>HHHHHHGSM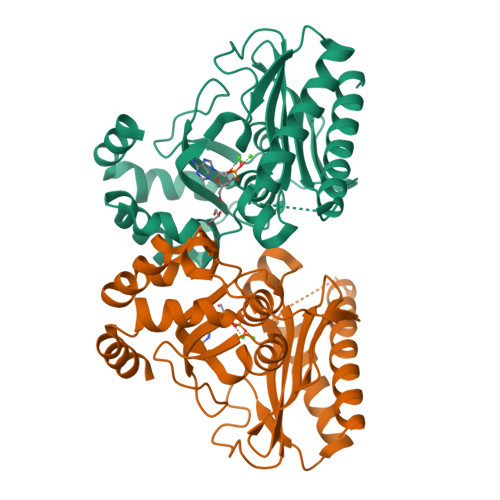ALYGFAQGLIQEAGIRIKQLMEQNLTIETKSNPNDLVTNVDKATEDFIFDTILETYPNHQVLGEEGHGHDIDTSKGTVWVVDPIDGTLNFVHQQENFAISIGIYIDGKPYAGFVYDVMADVLYHAKVGEGAYRGSQPLKPLNDSNLRQSIIGINPNWLTKPILGEIFKEIVNDSRSARAYGSAALEIVSVATGNLEAYMTPRLQPWDFAGGLVILYEVNGQASNLLGEPLTISGPNSILVGNRGLHQEISNDYLEPHHDALIQLHEQRFKRKSK[2x]>GAMHALGHCCTVVTTRGPSHWLLLLDTHLGTLPGFKVSAGRGLPAAEVYFEAGPRVSLSRTDATIVAVYQSILFQLLGPTFPASWTEIGATMPHNEYTFPRFISNPPQFATLAFLPLLSPTSPLDLRALMVTAQLMCDAKRLSDEYTDYSTLSASLHGRMVATPEISWSLYVVLGIDSTQTSLSYFTRANESITYMRYYATAHNIHLRAADLPLVAAVRLDDLKDHQIPAPGSWDDLAPKLRFLPPELCLLLPDEFDLIRVQALQFLPEIAKHICDIQNTICALDKSFPDCGRIGGERYFAITAGLRLDQGRGRGLAGWRTPFGPFGVSHTDVFQRLELLGDAVLGFIVTARLLCLFPDASVGTLVELKMELVRNEALNYLVQTLGLPQLAEFSNNLVAKSKTWADMYEEIVGSIFTGPNGIYGCEEFLAKTLMSPEHSKTVGSACPDAVTKASKRVCMGEAGAHEFRSLVDYACEQGISVFCSSRVSTMFLERLRDIPAEDMLDWYRLGIQFSHRSGLSGPGGVVSVIDIMTHLARG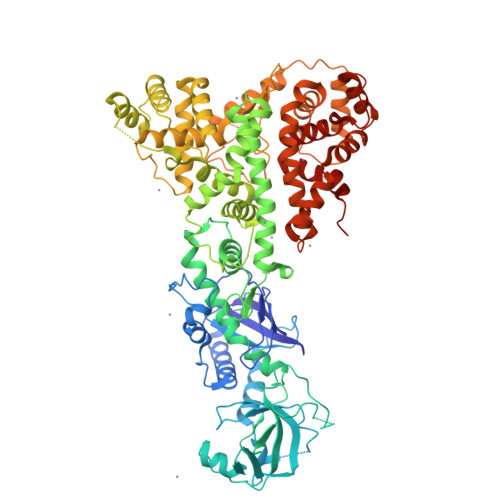LWLGSPGFYVEQQTDKNESACPPTIPVLYIYHRSVQCPVLYGSLTETPTGPVASKVLALYEKILAYESSGGSKHIAAQTVSRSLAVPIPSGTIPFLIRLLQIALTPHVYQKLELLGDAFLKCSLALHLHALHPTLTEGALTRMRQSAETNSVLGRLTKRFPSVVSEVIIESHPKIQPDSKVYGDTFEAILAAILLACGEEAAGAFVREHVLPQVVADA[4x]> GPDSMSDIKQLLKEAKQELTNRDYEETIEISEKVLKLDPDNYFAHIFLGKALSSLPASNNVSSNRNLERATNHYVSAAKLVPDNLLAWKGLFLLFRTTEVVPDILSYDEYFDLCGQYADALLKQEQSQVELINDIKLLKKTHPDCQKAFYQHLKPGSLMAETIGRHLSTPQDALLNLIKILSNIETTEIGKTLSQNRLKLKASDPDYQIKLNSFSWEIIKNSEIDQLYNQLVNILADDQKRSEIENQWLEYRIKVLKSMPLDVKKDFFTKVKEMVEDMVLVNHQSLLAWQKYFEWTDYEDLDNMDAPLIIKYFKKFPKDPLAMILYSWLSSKLSKYDIKSLESANKPPEGHKKTEKETDIKDVDETNEDEVKDRVEDEVKDRVEDEVKDQDEEAKEDEEEDLDDIEIGLLEEEVVTVLTENIVKCKNNILAHRILCQYYLLTKEYEAALPYIKNGISLIAYNIKDLGVHLPLTKREFSLDLATVYTYVDAPKDHNAALKLYDNILSGDFSNIQAKMG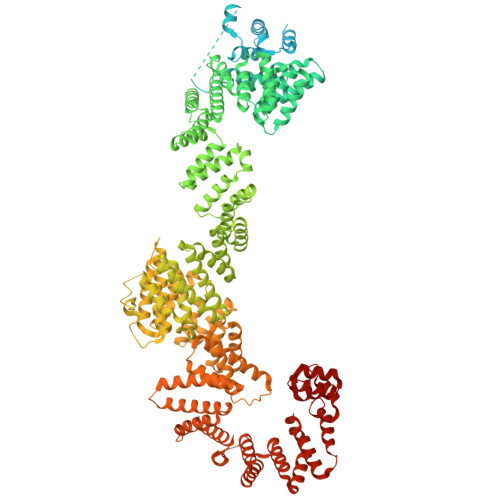KGIIFIERKNWKDAMTLLTQVHEQSPNNLEVLSELSWSKAHMGYMDEALAGLDTVIKGIKGMDLRSIDFRALNLWRQAKVYIMKHASINDAKQENVKCAFKLLIQSIKILDTFAPGFSTLGDIYCHYYKDHLRAFKCYFKAFDLDAGDYTAAKYITETYASKPNWQAASSIASRLIKGEKAKAELRSNNWPFRVVGIAHLEKQEESDSIEWFQSALRVDPNDVESWVGLGQAYHACGRIEASIKVFDKAIQLRPSHTFAQYFKAISLCDVGEYLESLDILEKVCQEAATEESFQIGLVEVLMRCSLDLYSQGFLLKSVSIAKDTIERIKIIISELKCENQQVWIYLSQVLRLFIWIESKVDTLPVESLVSIFENSQFSGSEEIDSVDNIKIDTLLDSTTDDNVSIACKFLILASKYSVSDQKFTDIAGTVRASYWYNIGISELTAFITLKEPQYRDAAIFAFKKSIQLQSNTSETWIGLGIATMDINFRVSQHCFIKATALEPKATNTWFNLAMLGLKKKDTEFAQQVLNKLQSLAPQDSSPWLGMALILEEQGDIIGSSKLFAHSFILSNGRSKAAQFMYAKNVLENHINNGDDERDIETVEKLTTASIALEQFFKKSPDSQFALQCALLTLERLHHYENANELANRLIGILEKKFEKTQDERELFNFAIIKGQFARIHLGLGNFELSIENADLSQGIISESSDEKSMKTKISNHICLGLSYFFLNDFDQTLNQFQELLSISKDSKHLVVLIAKVLYDVGESDTKEIALQELTEYIATSGADLLVTLTIAAMSILDDKREDLSIILEELKALPLSKQIIDKHKDAPYLIEEITKRLYRNDTGKQVWQRSAYFFPNNLKVWERLDKNIQRRIASNGQNKVTAEEMSKLYCESKNLRSIQRGMFLCPWNVTAVKALNECF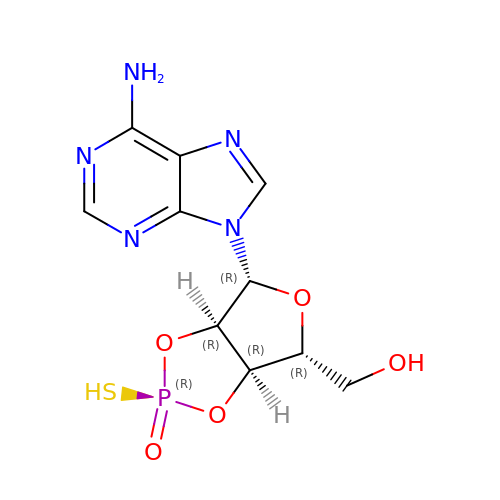[(3aR,4R,6R,6aR)-4-(6-aminopurin-9-yl)-2-oxidanylidene-2-sulfanyl-3a,4,6,6a-tetrahydrofuro[3,4-d][1,3,2]dioxaphosphol-6-yl]methanol | C10 H12 N5 O5 P S | OMSUUENXGWGOLC-PUHOFUEYSA-N benzyl (3S,5'R)-2-oxo-1,2-dihydrospiro[indole-3,3'-pyrrolidine]-5'-carboxylate | 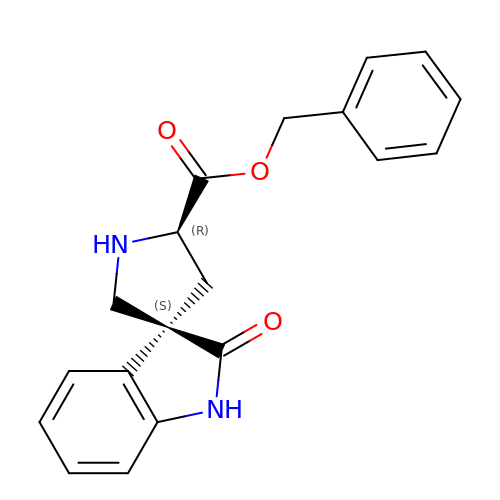C19 H18 N2 O3 | WDDNNMQSTPFSMZ-VQIMIIECSA-N> QT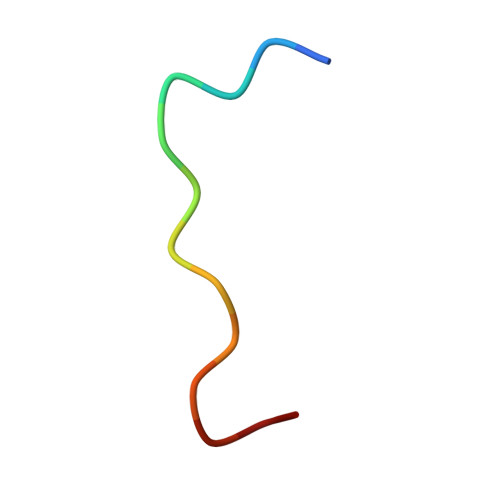AGANSQRGSAG> QEPVTVLRWDFEEIVGEQNVQALPAEWIASSKEGIAVERTEQGGRCLHVWVDAATGPGSRNIRYRLPVDKLRGQRVRVNALVRAKGVSQPPKPWNGIKCMLRIESGGEIQWPQQNLPGGDFDWRPIQFVVAVPDDCQQVDLIVGLENVTGDAWFDNIAVEVIPKKKLSSNHKEVFKGHNLPRLRGAMIGPHVTNADLLEFGNVWKANHIRWQLIWNGFPHSPADSATLDEYRQWLDGALKRLEAALPVCREAGILVTVDLHTPPGGRNEASECRIFHDREFQKAFIDIWEDIARRFADSDVVWGYDLVNEPVEGMVPDGLMNWQRLAEETARRVRAIDQKHAIIIEPAPWGSPSSIALLDPIDVPGVVYSVHMYVPHAFTHQGVYDNPVGIVYPGTIDGKWYDRNTLRKVLEPVRRFQEENGVHIYIGEFS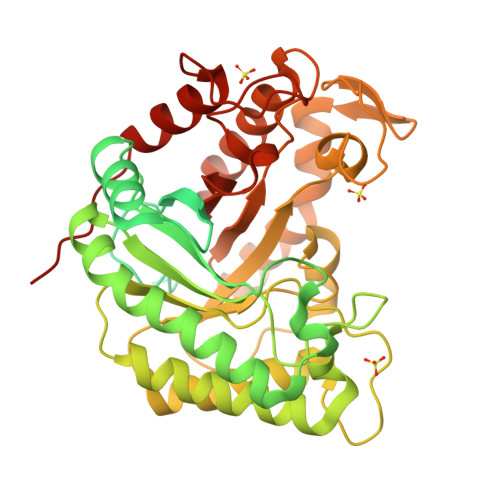AIRWAPADSACQYLKDCIEIFEEYGWDWAYHAFREWDGWSVEHGPDRNDRNRTATPTDRALLLRSWYAENVKPQFSDKKKD>AVTTRQITVPSAPMGWASWNSFAAKIDYSVIKKQVDAFVAAGLPAAGYTYINIDEGWWQGTRDSAGNITVDTAEWPGGMSAITAYIHSKGLKAGIYTDAGKDGCGYYYPTGRPAAPGSGSEGHYDQDMLQFSTWGFDFVKVDWCGGDAEGLDAATTYKSISDAVGRAAATTGRPLTLSICNWGYQNPWNWAAGQAPLWRTSTDIIYYGNQPSMTSLLSNFDQTLHPTAQHTGYYNDPDMLMVGMDGFTAAQNRTHMN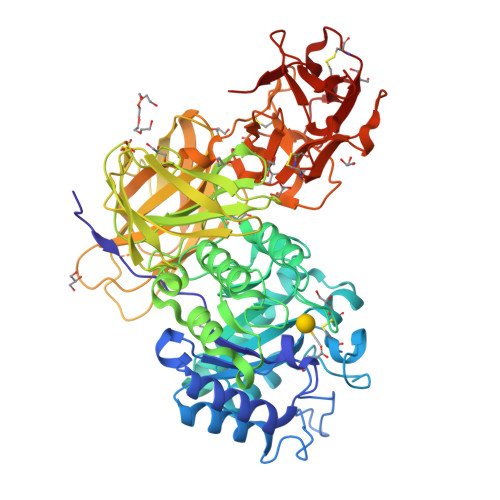LWAISGAPLLAGNDLTTMTSETAGILKNPEVIAVDQDSRGLQGVKVAEDTTGLQAYGKVLSGTGNRAVVLLNRTSAAHDITVRWSDLGLTNASATVRDLWARQNVGTSATGYTASVPAGGSVMLTVTGGTEAAGGAYAATSTGRYTGVTAASTGLNVVDVAYTNNTSSARTATLQVNGQTATTVSFPPTGASAGTVSVEVSLSKGSANTLALSGGPATEGITVRPLPGTNGALVTGKQSGRCADIYNNTITNGTQAELWDCNGGPNQSWTYTSRKELVLYGNKCLDAYNLGTTNGTKVVIWDCNGQANQKWNINSDGTITNVNAGLCLDAYNAATANGTSLVLWSCGTGDNQKWTVT[2x]> MILDTDYITEDGKPVIRIFKKENGEFKIDYDRNFEPYIYALLKDDSAIEDVKKITAERHGTTVRVVRAEKVKKKFLGRPIEVWKLYFTHPQDQPAIRDKIKEHPAVVDIYEYDIPFAKRYLIDKGLIPMEGDEELKMLAFAIATLYHEGEEFAEGPILMISYADEEGARVITWKNIDLPYVDVVSTEKEMIKRFLKVVKEKDPDVLITYNGDNFDFAYLKKRSEKLGVKFILGREG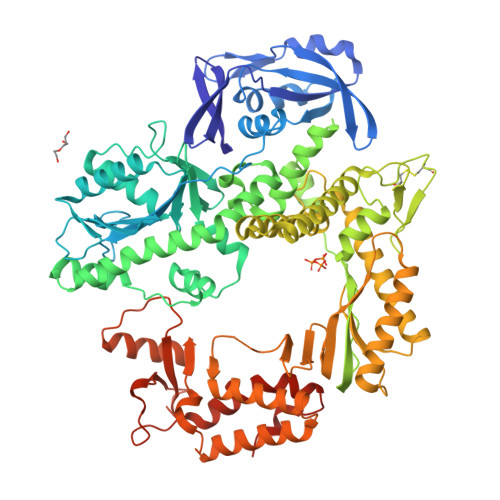SEPKIQRMGDRFAVEVKGRIHFDLYPVIRRTINLPTYTLEAVYEAIFGQPKEKVYAEEIAQAWETGEGLERVARYSMEDAKVTYELGKEFFPMEAQLSRLVGQSLWDVSRSSTGNLVEWFLLRKAYERNELAPNKPDERELARRRESYAGGYVKEPERGLWENIVYLDFRSLYPSIIITHNVSPDTLNREGCEEYDVAPQVGHKFCKDFPGFIPSLLGDLLEERQKVKKKMKATIDPIEKKLLDYRQRLIKILANSFYGYYGYAKARWYCKECAESVTAWGRQYIETTIREIEEKFGFKVLYADTDGFFATIPGADAETVKKKAKEFLDYINAKLPGLLELEYEGFYKRGFFVTKKKYAVIDEEDKITTRGLEIVRRDWSEIAKETQARVLEAILKHGDVEEAVRIVKEVTEKLSKYEVPPEKLVIYEQITRDLKDYKATGPHVAVAKRLAARGIKIRPGTVISYIVLKGSGRIGDRAIPFDEFDPAKHKYDAEYYIENQVLPAVERILRAFGYRKEDLRYQKTRQVGLGAWLKPKT4-amino-N-(6-chloro-2-fluoro-3-{[(pyrrolidin-1-yl)sulfonyl]amino}phenyl)quinazoline-8-carboxamide 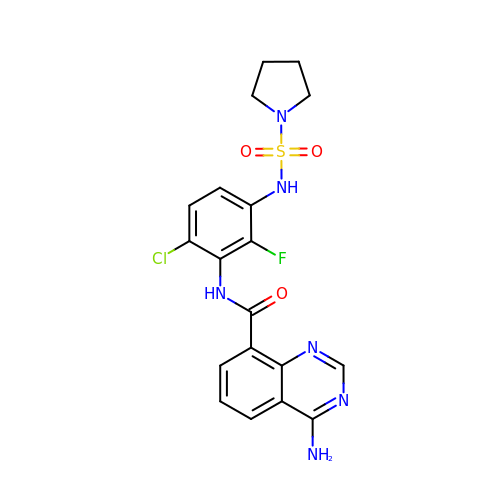| C19 H18 Cl F N6 O3 S | SKKINZODGXHKJJ-UHFFFAOYSA-N3-amino-7-chloro-2-nonylquinazolin-4(3H)-one 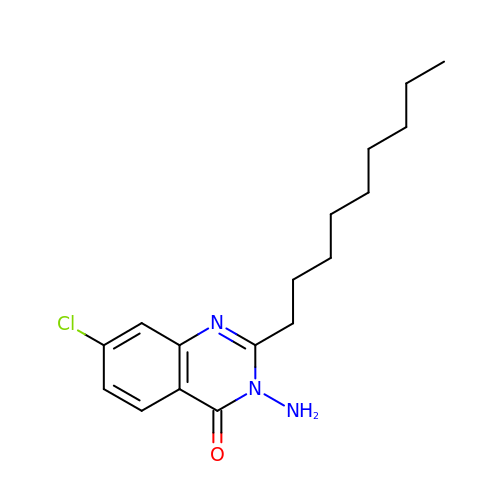| C17 H24 Cl N3 O | PLTFJOYTWYIUIG-UHFFFAOYSA-N DapE hydrolyzes N-succinyl-L,L-diaminopimelic acid to L,L-diaminopimelic acid and succinate, is part of a biosynthetic pathway that is the major source of lysine in bacteria, and is essential for cell growth and proliferation. All the DapE enzymes characterized to date belong to the M20 family of dinuclear Zn(II)-dependent metalloproteases. In order to examine the role of the catalytic domain of DapE enzymes and the role of the active site loops, we have engineered the HiDapE and the DapE from Vibrio cholerae (VcDapE) by deleting their dimerization domains. Removal of the dimerization domain in DapE enzymes renders the enzyme inactive, even though the resulting truncated proteins have structures of the catalytic domain that are remarkably similar to WT-DapE and AAP.

The monomeric state of VcDapET was confirmed by SEC (the estimated MW of 28.7 kDa) and DLS measurements (the estimated average MW of 23.2 kDa). Two VcDapET structures were determined, the apo- and the dinuclear Zn(II)-loaded form. The final models for both apo- and Zn(II)-loaded VcDapET included two molecules of the catalytic domain in the asymmetric unit. The two V. cholerae structures are virtually identical and superimpose with the average rmsd of 0.25 Å for 265 equivalent Cα atoms suggesting that binding of Zn(II) does not induce any major structural changes. Since the structures of VcDapET were determined in both the apo- and dinuclear Zn(II)-loaded forms, it is evident that removal of either the dimerization domain or the metal cations does not alter the overall structure of the catalytic domain. Similarly to HiDapET, the most flexible regions of the protein are Region I and Region II. Region I corresponds to the engineered loop (the connector) where the deleted dimerization domain is replaced with two glycines. Region II (residues 210–224) forms a loop overhanging the active site metal ions, which includes residues 211–213 that form part of loop V (vide infra). A change is observed in loop V, which in VcDapET adopts a conformation that is significantly different from the one observed for WT-HiDapE (in HiDapET this loop is disordered). Interestingly, this loop is also partially disordered in the structure of HiDapET, while in VcDapET structures its conformational flexibility is signified by the double conformation of the main chain Gly 213 (peptide flip).

>[2x]SNATDSPVLALAKELISRQSVTPADAGCQDLMIERLKALGFEIESMVFEDTTNFWARRGTQSPLFVFAGHTDVVPAGPLSQWHTPPFEPTVIDGFLHGRGAADMKGSLACMIVAVERFIAEHPDHQGSIGFLITSDEEGPFINGTVRVVETLMARNELIDMCIVGEPSSTLAVGDVVKNGRRGGGFLTDTGELLAAVVAAVEEVNHQAPALLTTGGTSDGRFIAQMGAQVVELGPVNATIHKVNECVRIADLEKLTDMYQKTLNHLLG> GAMDPMIVLGLEGTAHTISCGIIDESRILAMESSMYRPKTGGIRPLDAAVHHSEVIDTVISRALEKAKISIHDIDLIGFSMGPGLAPSLRVTATAARTISVLTGKPIIGVNHPLGHIEIGRRVTGAIDPVMLYVSGGNTQVIAHVNGRYRVLGETLDIGIGNMIDKFAREAGIPFPGGPEIEKLAMKGTKLLDLPYSVKGMDTAFSGILTAALQYLKTGQAIEDISYSIQETAFAM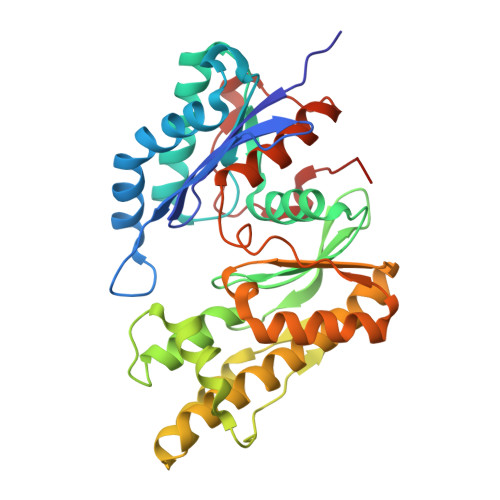LVEVLERALYVSGKDEILMAGGVALNRRLRDMVTNMAREAGIRSYLTDREYCMDNGIMIAQAALLMYKSGVRMSVEETAVNPRFRIDEVDAPWITDAS> RSSQLPAPQHPKIRLYNAEQVLSWEPVALSNSTRPVVYQVQFKYTDSKWFTADIMSIGVNCTQITATECDFTAASPSAGFPMDFNVTLRLRAELGALHSAWVTMPWFQH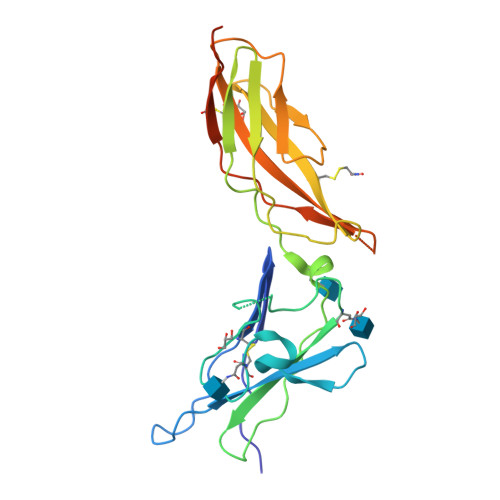YRNVTVGPPENIEVTPGEGSLIIRFSSPFDIADTSTAFFCYYVHYWEKGGIQQVKGPFRSNSISLDNLKPSRVYCLQVQAQLLWNKSNIFRVGHLSNISCYETMADASTELQQTGHHHHHHE>GSKVVKFSYMWTINNFSFCREEMGEVIKSSTFSSGANDKLKWCLRVNPKGLDEESKDYLSLYLL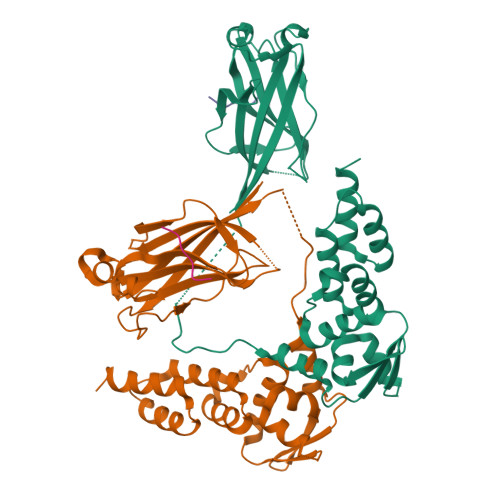LVSCPKSEVRAKFKFSILNAKGEETKAMESQRAYRFVQGKDWGFKKFIRRGFLLDEANGLLPDDKLTLFCEVSVVQDSVNISGQNTMNMVKVPECRLADELGGLWENSRFTDCCLCVAGQEFQAHKAILAARSPVFSAMFEHEMEESKKNRVEINDVEPEVFKEMMCFIYTGKAPNLDKMADDLLAAADKYALERLKVMCEDALCSNLSVENAAEILILADLHSADQLKTQAVDFINYHATDVLETSG[2x];>DEVTSTT[2x]>[4x]APMKLYGAVMSWNLTRCATALEEAGSDYEIVPINFATAEHKSPEHLVRNPFGQVPALQDGDLYLFESRAICKYAARKNKPELLREGNLEEAAMVDVWIEV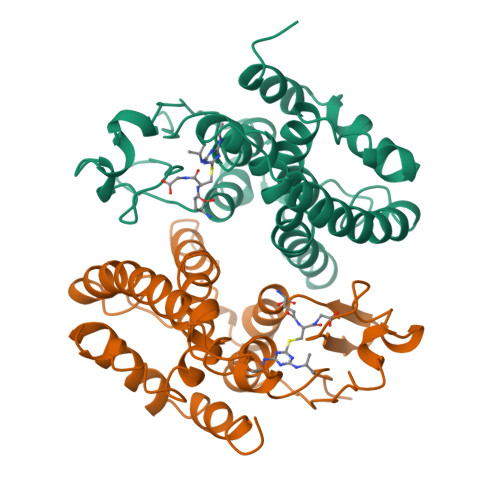EANQYTAALNPILFQVLISPMLGGTTDQKVVDENLEKLKKVLEVYEARLTKCKYLAGDFLSLADLNHVSVTLCLFATPYASVLDAYPHVKAWWSGLMERPSVQKVAALMKPSA>[3x]MGSDKIHHHHHHMKILITGANGQLGREIQKQLKGKNVEVIPTDVQDLDITNVLAVNKFFNEKKPNVVINCAAHTAVDKCEEQYDLAYKINAIGPKNLAAAAYSVGAEIVQISTDYVFDGEAKEPITEFDEVNPQSAYGKTKLEGENFVKALNPKYYIVRTAWLYGDGNNFVKTMI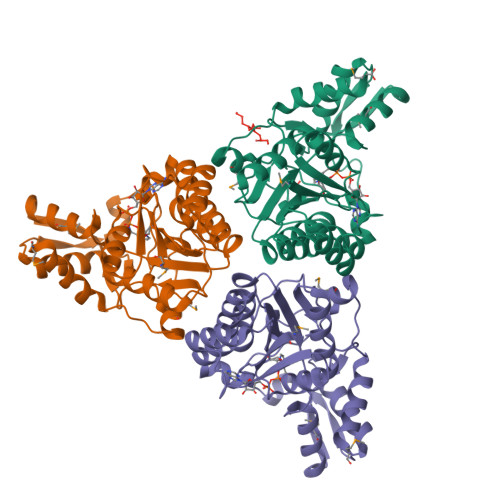NLGKTHDELKVVHDQVGTPTSTVDLARVVLKVIDEKNYGTFHCTCKGICSWYDFAVEIFRLTGIDVKVTPCTTEEFPRPAKRPKYSVLRNYMLELTTGDITREWKESLKEYIDLLQM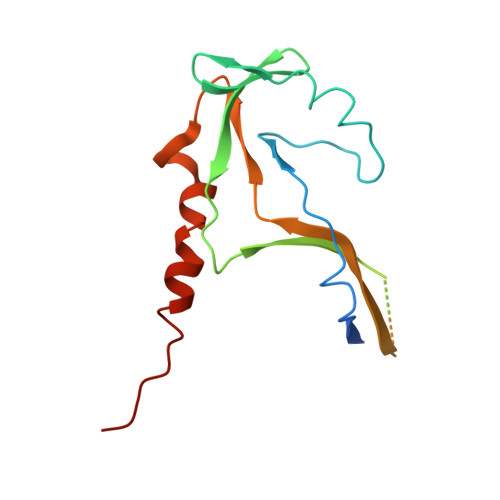> MESGDEAAIERHRVHLRSATLRDAVPATLHLLPCEVAVDGPAPVGRFFTPAIRQGPEGLEVSFRGRCLRGEEVAVPPGLVGYVMVTEEKKVSMGKPDPLRDSGTDDQEEEPLERDFDRFIGATANFSRFTLWGLETIPGPDAKVRGALTWPSLAAAIHAQVPED> GTACG;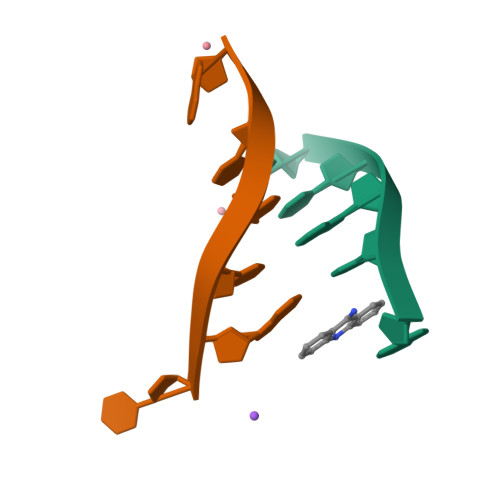> CGTACG> RTITGDTCNEETQNLSTIYLREYQSKVKRQIFSDYQSE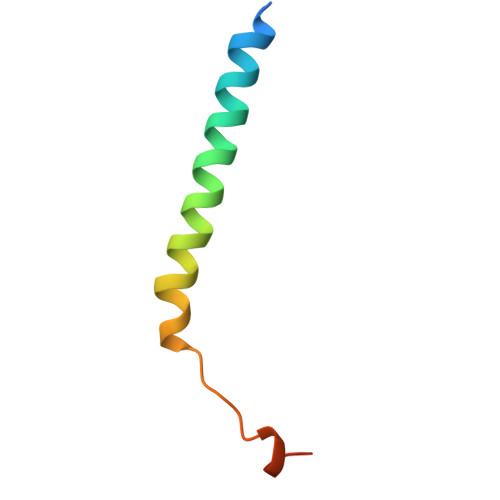VDIYNRIRDEL4-[3-CARBOXYMETHYL-3-(4-PHOSPHONOOXY-BENZYL)-UREIDO]-4-[(3-CYCLOHEXYL-PROPYL)-METHYL-CARBAMOYL]BUTYRIC ACID | C25 H38 N3 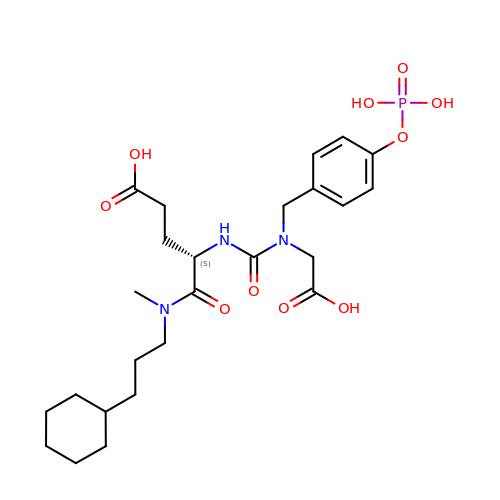O10 P | JSBQUMXQEBZYPW-NRFANRHFSA-N> LGGDRDFWLQVGIDPIQIMTGTATFYTLRCYLDDRPIFLGRNGRISVFGSERALARYLADEHDHDLSDLSTYDDIRTAATDGSLAVAVTDDNVYVLSGLVDDFADGPDAVDREQLDLAVELLRDIGDYSEDSAVDKALETTRPLGQLVAYVLDPHSVGKPTAPYAAAVREW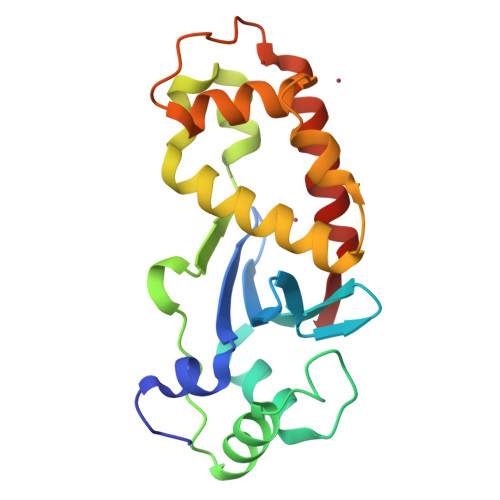EKLERFVESRLRRE octyl 1-thio-beta-D-glucopyranoside | 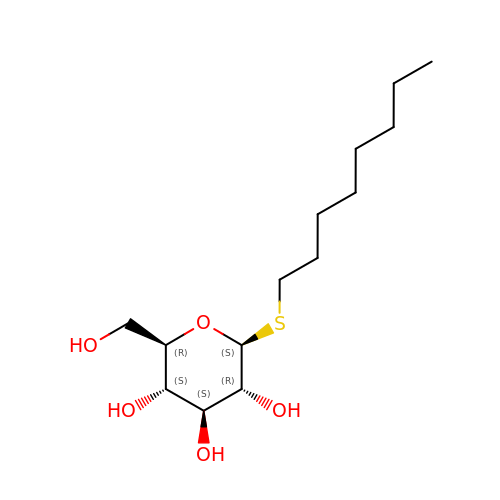C14 H28 O5 S | CGVLVOOFCGWBCS-RGDJUOJXSA-N> PPCLDSELTEFPLRMRDWLKNVLVTLYERDEDNNLLTEKQKLRVKKIHENEKRLEAGDHPVELLARDFEKNYNMYIFPVHWQFGQLDQHPIDGYLSHTELAPLRAPLIPMEHCTTR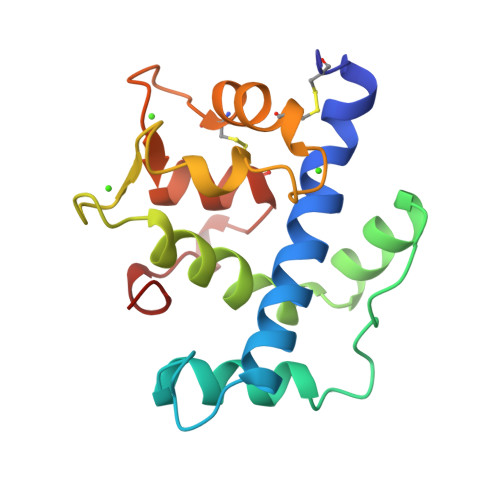FFETCDLDNDKYIALDEWAGCFGIKQKDIDKDLVI>[2x]GAMAPLTQDRIVVTALGILDAEGLDALSMRRLAQELKTGHASLYAHVGNRDELLDLVFD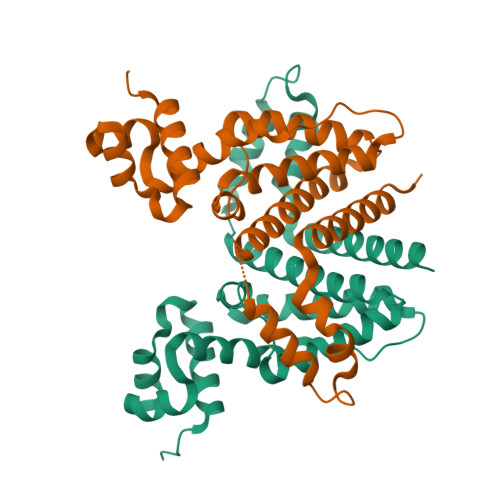IVLTEVEVPEPEPGRWAEQVKEMCRSLRRMFLAHRDLARIAIDRVPLGPNGMVGMERTMNLLRSGGLHDELAAYGGDLLSTFVTAEALEQSSRNPGTEQGREQAGVFADQLHGYLKSLPATSFPNLVHLAGPITSLDSDRRFELGLEIIIAGLLAGAGEAADDQVRTAGSPPAES>[8x]MGSSHHHHHHENLYFQGMTSIGKQRGLARLADEDGHFTMVALDQRPPLLQALAKARGIPADQVEFADMLAAKRLLVEALAHDASSMLLDPNFAMPA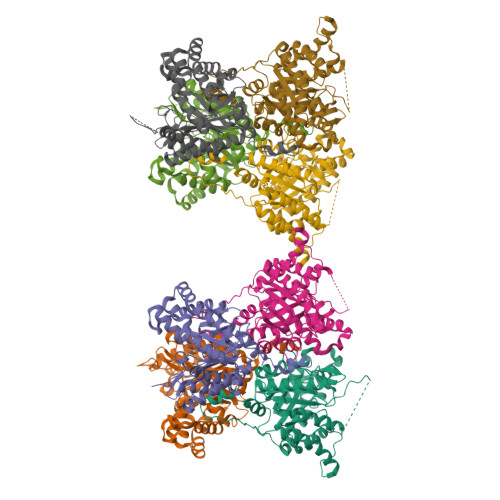AIDVLPARTGLIVTLEEHRFQDTPGGRKSRSIDNWSVEKIRRVGGDAVKVLAWYRPDASDEVLQHQKDYVRTIGAECRRHDIPYVLELLVYPFPDSDRHTTDYVESADKRADLVIESVREFAKPEYGVDLYKLETPLPAASLPPMDDSAESRAAAAQFAEVGSICADAGIPWVLLSGGAAPEQFERVLSYSYAAGAQGFLAGRTIWLDAVQNHFPDREAVLTALKGDGMKILKDLGRLTREKAQPWKPDFRLEQVDREGAFSCAYA> QDVRVRVLPEVRGRLGGTVELPCHLLPPTTERVSQVTWQRLDGTVVAAFHPSFGVDFPNSQFSKDRLSFVRARPETNADLRDATLAFRGLRVEDEGNYTCEFATFPNGTRRGVTWLRVIAQPENHAEAQEVTIGPQSVAVARCVSTGGRPPARITWISSLGGEAKDTQEPGIQ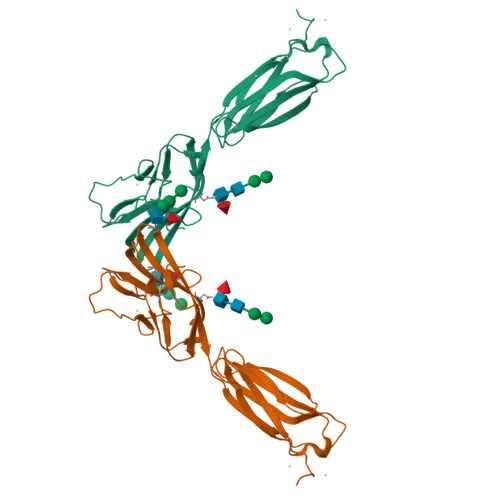AGTVTIISRYSLVPVGRADGVKVTCRVEHESFEEPILLPVTLSVRYHHHHHH> MAMQAAKRANIRLPPEVNRILMIRNLPYKITAEEMYDIFGKYGPIRQIRV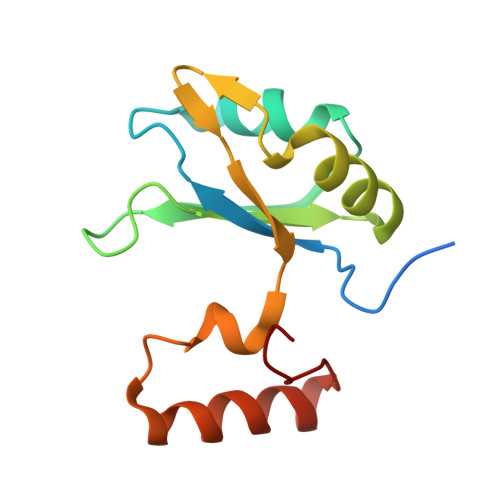GNTPETRGTAYVVYEDIFDAKNACDHLSGFNVCNRYLVVLYYNANRAFQKMDTKKKEEQLKLLKEKYGINTDPPK> ANKGFLEEVRKGNLERECLEEPCSREEAFEALESLSA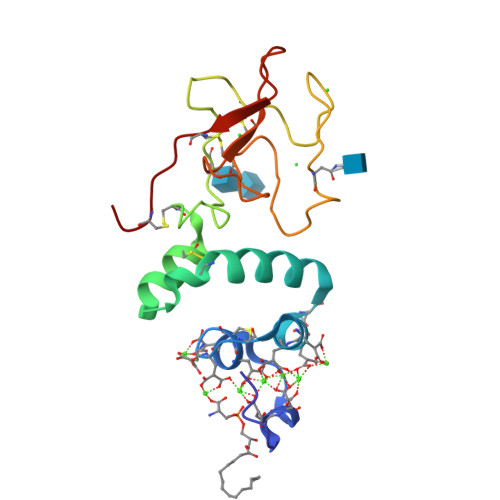TDAFWAKYTACESARNPREKLNECLEGNCAEGVGMNYRGNVSVTRSGIECQLWRSRYPHKPEINSTTHPGADLRENFCRNPDGSITGPWCYTTSPTLRREECSVPVCGQ> SVRDELRWVF;> VSYANAVSRAAPAVANLYTTKMVSKPSHPLFDDPMFRRFFGDNLPQQKRMESSLGSAVIMSAEGYLLTNNHVTAGADQIIVALRDGRETIAQLVGSDPETDLAVLKIDLKNLPAMTLGRSDGIRTGDVCLAIGNPFGVGQTVTMGIISATGRNQLGLNTYEDFIQTDAAINPGNAGGALVDAAGNLIGINTAIFSKSGGSQGIGFAIPTKLALEVMQSIIEHGQVIRGWLGVEVKALTPELAESLGLGETAGIVVAGVYRDGPAARGGLLPGDVILTIDKQEASDGRRSMNQVARTRPGQKISIVVLRNGQKVNLTAEVGLRPPPAPAP

AlgW, a membrane-bound periplasmic serine protease belonging to the HtrA protein family, is a key regulator of the regulated intramembrane proteolysis (RIP) pathway and is responsible for transmitting the envelope stress signals in Pseudomonas aeruginosa. The AlgW PDZ domain senses and binds the C-terminal of mis-localized outer membrane proteins (OMPs) or periplasmic protein MucE, leading to catalytic activation of the protease domain. HtrA protease is characterized by its trypsin-like catalytic domain and regulatory PDZ domain; the catalytic triad was surrounded by several loops (L1, L2, L3, LD, LA) but, usually, in an inactive mode, and could be activated by sensing a specific molecular stimulus. The catalytic triad (H123, D153, and S227) sites are located between two β-barrels and are surrounded by activation loops L1 to L3, LD, and LA (named according to DegS nomenclature).

In order to elucidate the structural basis of the AlgW reaction mechanism, we prepared the periplasmic soluble domain of AlgW and its inactive mutant AlgWS227A. Protein samples were mixed with two types of peptide activator (tripeptide WVF, decapeptide SVRDELRWVF) prior to crystallization trials, yielding four complex structures, AlgW-tripeptide, AlgWS227A-tripeptide, AlgW-decapeptide, and AlgWS227A-decapeptide, with resolutions from 1.8 to 2.6 Å. AlgWS227A-decapeptide could even generate a DegQ-like “cage” architecture after symmetry operation; the dodecamer of soluble AlgW contains four trimers, with the 12 LA loops protruding toward the interior of the cage. LA-mediated higher oligomerization is an important regulation mechanism in the HtrA family; however, very few close contacts are observed between trimers in AlgW-decapeptide and AlgWS227A-decapeptide structures, indicating that crystal packing may, in fact, dominate the above-described intertrimer associations. Fortunately, LA loops could be reliably modeled in AlgW-decapeptide and AlgWS227A-decapeptide structures, allowing us to explore the conformational regulation mode of the LA loop. By comparing the two sets of decapeptide-bound structures, we found that the LA loop shows joint angle shifts of about 7.65 degrees. It seems that the LA loop in the AlgWS227A-decapeptide structure represents the major state of LA, because similar to the LA loops in tripeptide-bound structures, they all need to stabilize the antiparallel β1-β4 sheet by forming main-chain hydrogen between D129-Q130 and T72 and maintain the orientation of β1 through the weak interaction between T71 and V124. Consistently, AlgW-peptide bound structures also demonstrated different interdomain orientations, in which the joint angles of the PDZ relative to the protease domain are AlgW-WVF (25.62°) < AlgWS227A-WVF (25.74°) < AlgW-decapeptide (25.47 to 26.48°; average, 26.13°) < AlgWS227A-decapeptide (26.65°).>GYSSEKIPVTGSGFVAKDDSL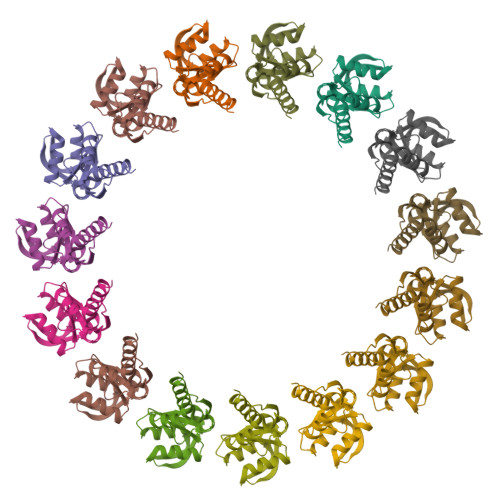RTFFDAMALQLKEPVIVSKMAARKKITGNFEFHDPNALLEKLSLQLGLIWYFDGQAIYIYDASEMRNAVVSLRNVSLNEFNNFLKRSGLYNKNYPLRGDNRKGTFYVSGPPVYVDMVVNAATMMDKQNDGIELGRQ[15x]>[2x]APTSSSTKKTQLQLEHLLLDLQMILNGINNYKNPKLTRMLTFKFYMPKK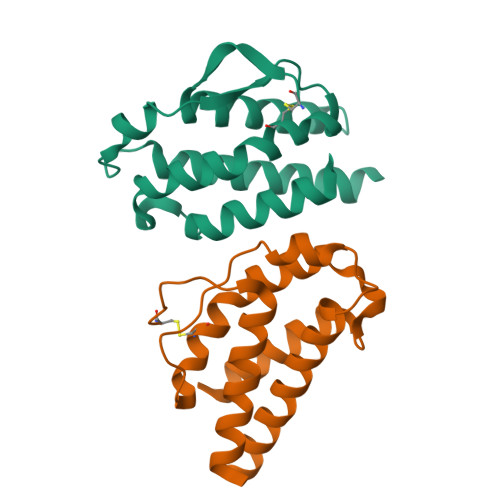ATELKHLQCLEEELKPLEEVLNLAQSKNFHLRPRDLISNINVIVLELKGSETTFMCEYADETATIVEFLNRWITFAQSIISTLT1-[3-[2-(1H-indol-3-yl)ethylsulfamoyl]phenyl]-3-(1,3-thiazol-2-yl)urea 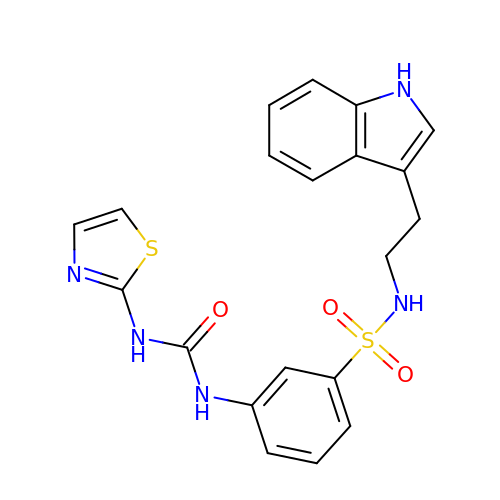| C20 H19 N5 O3 S2 | NYYVMDXWTXBRNW-UHFFFAOYSA-N> MLDLFTLSFSPDLSIASEAEQLTLQSKDDRLILEHPQPGLRTALEQLKQGNLTLAQLTE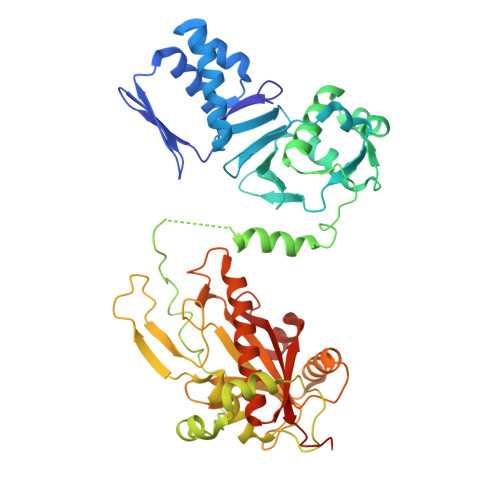LVSEQDGVEAGITFASELEKLVDLGWICHSVLPLITAIPIAKDYELNVPDSSWQTTAIALSRFAFLHQDLQQLVLESPRSKSKLVILDWRVGAVIAKLAQSDRGFIFATSADSLLADLSLELEELKRLFALLIATQMMDLEPEDETITQWKFHNLLFHHYTRLGRLDNSRKLNLPVFEHRDRYPYVKPVISTQAIPLVKPDLTALATTDMTLTEAIETRRSIREYSDQPITLAQLGEFLYRCARVKAVYTLPEDPMQVGESTTRPYPSGGALYELEIYPLVHQCGDLAAGLYHYQPLSHTLHPVADWTPEVESLVYDAWRATGQQSIPQIVLIITARFGRLFWKYHDIAYSLILKHVGVLYQTFYLVATAMQLAPSAIGAGNTTKFCQIAGLNPDEEASVGEFSLGAAKPQQQS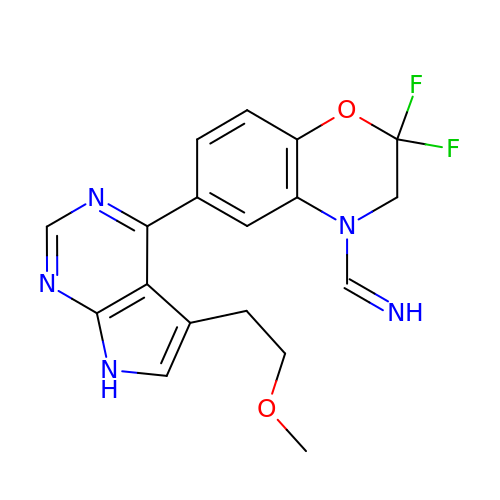(Z)-1-{2,2-difluoro-6-[5-(2-methoxyethyl)-7H-pyrrolo[2,3-d]pyrimidin-4-yl]-2,3-dihydro-4H-1,4-benzoxazin-4-yl}methanimine | C18 H17 F2 N5 O2 | YVXZGNOOOFSANU-NKVSQWTQSA-N> SMSRSKRDNNFYSVEIGDST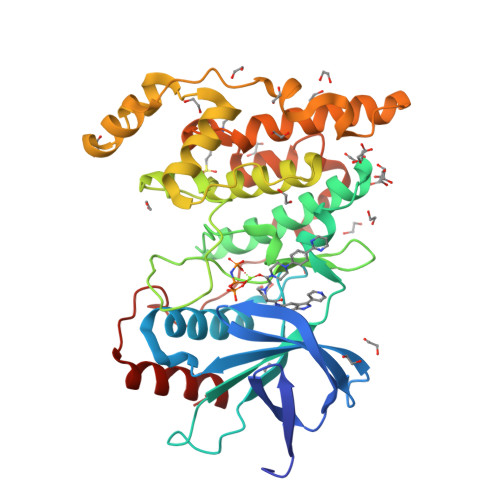FTVLKRYQNLKPIGSGAQGIVCAAYDAILERNVAIKKLSRPFQNQTHAKRAYRELVLMKCVNHKNIIGLLNVFTPQKSLEEFQDVYIVMELMDANLCQVIQMELDHERMSYLLYQMLCGIKHLHSAGIIHRDLKPSNIVVKSDCTLKILDFGLARTAGTSFMMTPYVVTRYYRAPEVILGMGYKENVDLWSVGCIMGEMVCHKILFPGRDYIDQWNKVIEQLGTPCPEFMKKLQPTVRTYVENRPKYAGYSFEKLFPDVLFPADSEHNKLKASQARDLLSKMLVIDASKRISVDEALQHPYINVWYDPSEAEAPPPKIPDKQLDEREHTIEEWKELIYKEVMDL> GAMDGTAAEPRPGAGSLQHAQPPPQPRKKRPEDFKFGKILGEGSFSTVVLARELATSREYAIKILEKRHIIK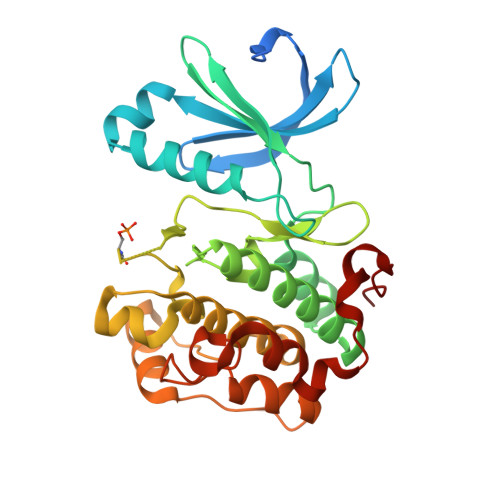ENKVPYVTRERDVMSRLDHPFFVKLYFTFQDDEKLYFGLSYAKNGELLKYIRKIGSFDETCTRFYTAEIVSALEYLHGKGIIHRDLKPENILLNEDMHIQITDFGTAKVLSPESKQARANSFVGTAQYVSPELLTEKSACKSSDLWALGCIIYQLVAGLPPFRAGNEGLIFAKIIKLEYDFPEKFFPKARDLVEKLLVLDATKRLGCEEMEGYGPLKAHPFFESVTWENLHQQTPPKLT(R)-1-(4-(4-(HYDROXYMETHYL)-1,3,2-DIOXABOROLAN-2-YL)PHENYL)GUANIDINE 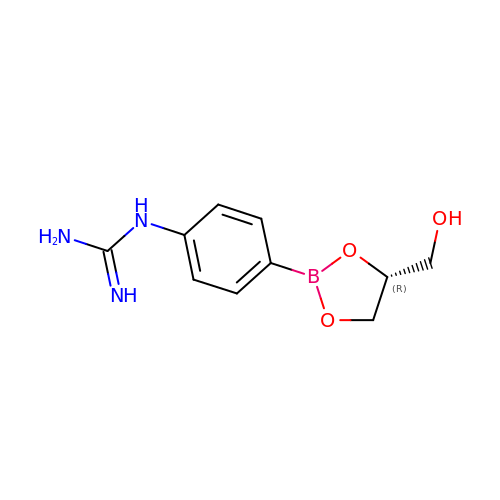| C10 H14 B N3 O3 | PTRUIYBNRUNGLM-SECBINFHSA-N>STQTQSSCSVPSAQEPLVNGIQVLMENSVTSSAYPNPSILIAMNLAGAYNLKAQKLL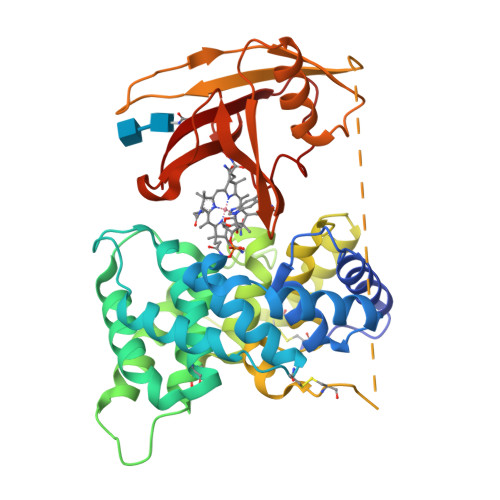TYQLMSSDNNDLTIGHLGLTIMALTSSCRDPGDKVSILQRQMENWAPSSPNAEASAFYGPSLAILALCQKNSEATLPIAVRFAKTLLANSSPFNVDTGAMATLALTCMYNKIPVGSEEGYRSLFGQVLKDIVEKISMKIKDNGIIGDIYSTGLAMQALSVTPEPSKKEWNCKKTTDMILNEIKQGKFHNPMSIAQILPSLKGKTYLDVPQVTCSPDHEVQPTLPSNPGPGPTSASNITVIYTINNQLRGVELLFNETINVSVKSGSVLLVVLEEAQRKNPMFKFETTMTSWGLVVSSINNIAENVNHKTYWQFLSGVTPLNEGVADYIPFNHEHITANFTQY[4x]> MNAVEIQGVSQRYGSMTVLHDLNLNLGEGEVLGLFGHNGAGKTTSMKLILGLLSPSEGQVKVLGRAPNDPQVRRQLGYLPE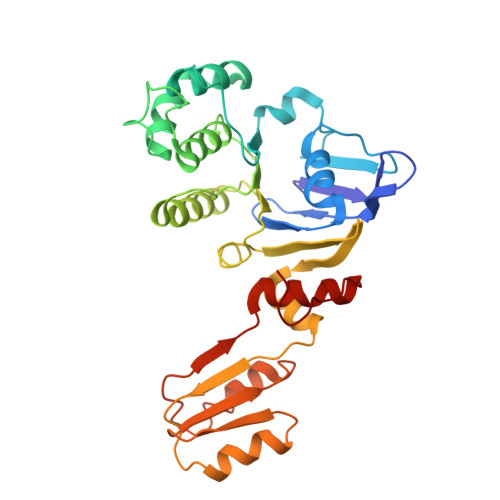NVTFYPQLSGRETLRHFARLKGAALTQVDELLEQVGLAHAADRRVKTYSKGMRQRLGLAQALLGEPRLLLLDEPTVGLDPIATQDLYLLIDRLRQRGTSIILCSHVLPGVEAHINRAAILAKGCLQAVGSLSQLRAEAGLPVRIRASGISERDSWLQRWTDAGHSARGLSESSIEVVAVNGHKLVLLRQLLGEGEPEDIEIHQPSLEDLYRYYMERAGDVRAQEGRL>[18x]CLTAPPKEAARPTLMPRAQSYKDLTHLPAPTGKIFVSVYNIQDETGQFKPYPASNFS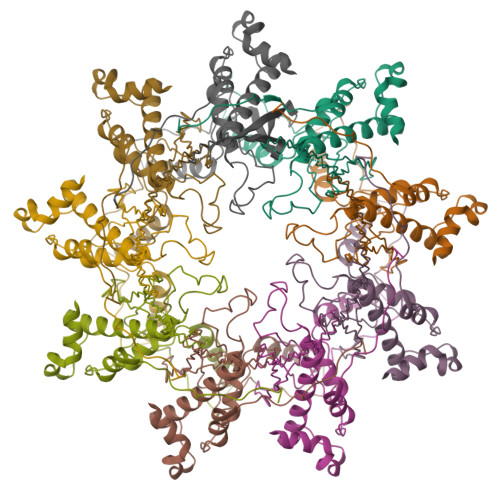TAVPQSATAMLVTALKDSRWFIPLERQGLQNLLNERKIIRAAQENGTVAINNRIPLQSLTAANIMVEGSIIGYESNVKSGGVGARYFGIGADTQYQLDQIAVNLRVVNVSTGEILSSVNTSKTILSYEVQAGVFRFIDYQRLLEGEVGYTSNEPVMLCLMSAIETGVIFLINDGIDRGLWDLQNKAERQNDILVKYRHMSVPPES2-(2-HYDROXY-PHENYL)-3H-BENZOIMIDAZOLE-5-CARBOXAMIDINE 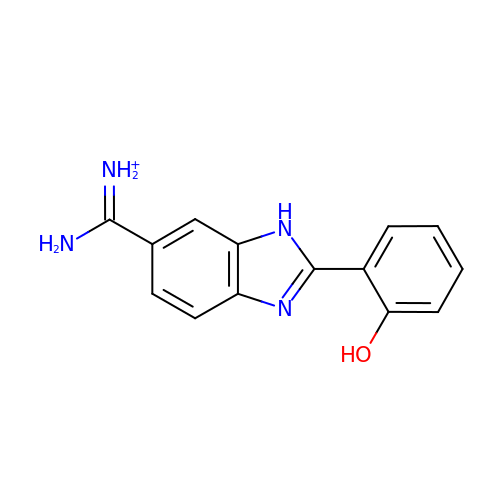| C14 H13 N4 O | URJKRCBBKTXOHS-UHFFFAOYSA-O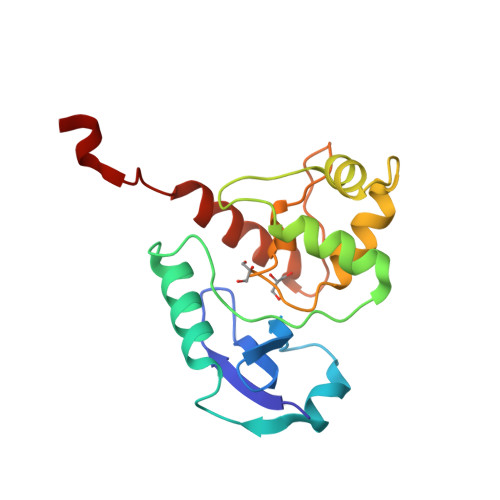> MVHYRTIDSPIGPLTLAGHGSVLTNLRMLEQTYEPSRTHWTPDPGAFSGAVDQLNAYFAGELTEFDVELDLRGTDFQQRVWKALLTIPYGETRSYGEIADQIGAPGAARAVGLANGHNPIAIIVPCHRVIGASGKLTGYGGGINRKRALLELEKSRAPADLTLFD> ATPHNSAQVGDFAETVLMCGDPLRAKLIAETYLENPKLVNNVRGIQGYTGTYKGKPISVMGHGM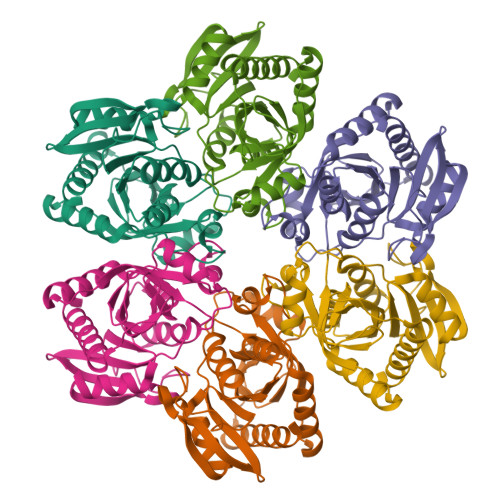GLPSICIYAEELYSTYKVKTIIRVGTCGAIDMDIHTRDIVIFTSAGTNSKINRIRFMDHDYPATASFDVVCALVDAAKELNIPAKVGKGFSTDLFYNPQTELAQLMNKFHFLAVEMESAGLFPIADLYGARAGCICTVSDHILHHEETTAEERQNSFQNMMKIALEAAIKL4-[5-oxidanyl-2-phenyl-1-[4-(4-propan-2-ylpiperazin-1-yl)phenyl]pent-1-enyl]phenol 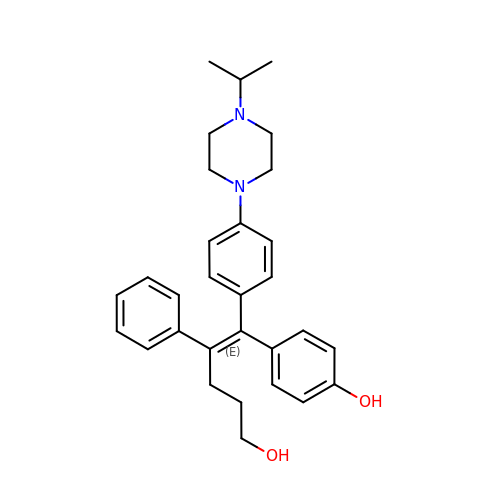| C30 H36 N2 O2 | RUUIHSHMHGOGMZ-QVIHXGFCSA-N> GSAMGSSSSDIQTKLKWSWSTSVFHPESNQVMAAPIVVQLNDDNGDGKIDEKDVADIIVVTFEGNKYANGGYIRALSGVDGSELWSYSNGGVIADARYAPAAADLDGDGLIEIVSTSALTPYINILDHQGNIKKQLLKSASGWRSVGDIALADINGDGNIEILAADGVYSYESGLLFSHDWAPSSIAFDSNGDGQREVFANGTLYQNNGAYLWQYQANDTVWFSSVANLDGDDKPELVVSVPASLSTPENSEIAVLEHDGSVKWRVNNLSNPGGSVQAVSSFLGKPSSSATTVDAQSAVYGYTDWAHQQRVLAENHQLAIRSGAVVDAIGANSQNMIGGSGGSLSTIDTSKVRAIDVTYGKNKYTWKYGVLEMSFTLDNGAKVTVGSKDSAFTSTTVRYDIPQGSQLLGMNVWSKEKHLFKHKQQVNAVQFLVGKVTADQSHMGIVYAGYYAVDMYDAQGNKVWS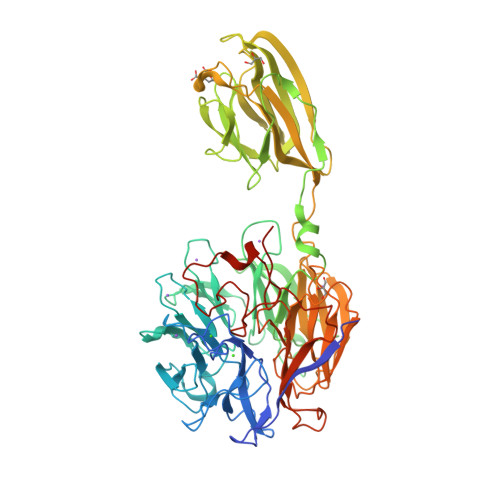VANDDLNSGKIGVSAYDFTGDGIDEVLVQDRLRMRILDGQTGRVMGIIANSSGTLWEYPVVADLEGNNNASLIMVANDYDRESQVNHGVFVYESANPSKPWRNATRIWNQYAFNFSDINANGTIPTNAQPSWLTHNSFRSATIRVPLK> MLRDLFDRAVVLSHYIHNLSSEMFSEFDKRYTHGRGFITKAINSCHTSSLATPEDKEQAQQMNQKDFLSLIVSILRSWNEPLYHLVTEVRGMQEAPEAILSKAVEIEEQTKRLLERMELIVSQVHPETKENEIYPVWSGLPS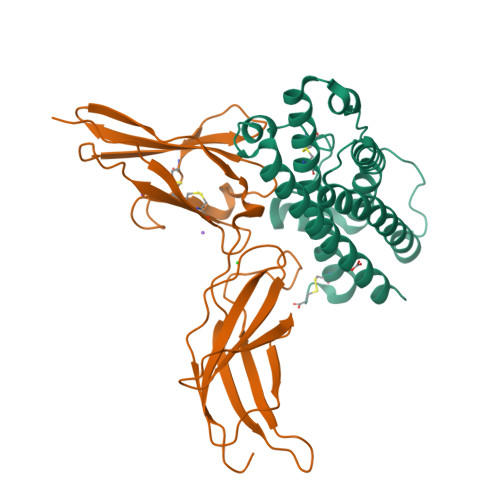LQMADEESRLSAYYNLLHCLRRDSAKIDNYLKLLKCRIIHNNNC;> MLPPGKPEIFKCRSPNKETFTCWWRPGTDGGLPTNYSLTYHREGETLMHECPDYITGGPNSCHFGKQYTSMWRTYIMMVNATNQMGSSFSDELYVDVTYIVQPDPPLELAVEVKQPEDRKPYLWIKWSPPTLIDLKTGWFTLLYEIRLKPEKAAEWEIHFAGQQTEFKILSLHPGQKYLVQVRCKPDHGYWSAWSPATFIQIPSDFTMND(3S,3'S)-N~1~,N~1~'-butane-1,4-diyldibutane-1,3-diamine | C12 H30 N4 | 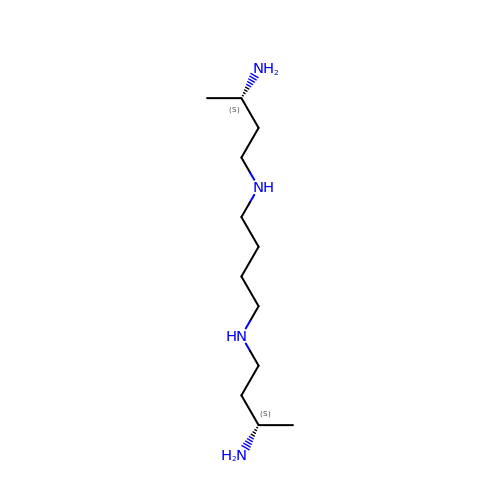LXKFTCVCBKNJNM-RYUDHWBXSA-N> GAMQGEVSKAASADSTTEGTPADGFTVLSTKSLFLGQKLQVVQADIASIDSDAVVHPTNTDFY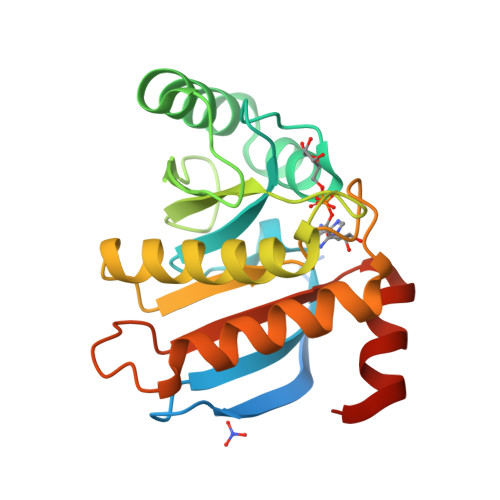IGGEVGNTLEKKGGKEFVEAVLELRKKNGPLEVAGAAVSAGHGLPAKFVIHCNSPVWGADKCEELLEKTVKNCLALADDKKLKSIAFPSIGSGRNGFPKQTAAQLILKAISSYFVSTMSSSIKTVYFVLFDSESIGIYVQEMAKLDAN> MADTQYILPNDIGVSSLDCREAFRLLSPTERLYAYHLSRAAWYGGLAVLLQTSPEAPYIYALLSRLFRAQDPDQLRQHALAEGLTEEEYQAFLVYAAGVYSNMGNYKSFGDTKFVPNLPKEKLERVILGSEAAQQHPEEVRGLWQTCGELMFSLEPRLRHLGLGKEGITTYFSGNCTMEDAKLAQDFLDSQNLSAYNTRLFKEVDGEGKPYYEVRLASVLGSEPSLDSEVTSKLKSYEFRGSPFQVTRGDYAPILQKVVEQLEKAKAYAANSHQGQMLAQYIESFTQGSIEAHKRGSRFWIQDKGPIVESYIGFIESYRDPFGSRGEFEGFVAVVNKAMSAKFERLVASAEQ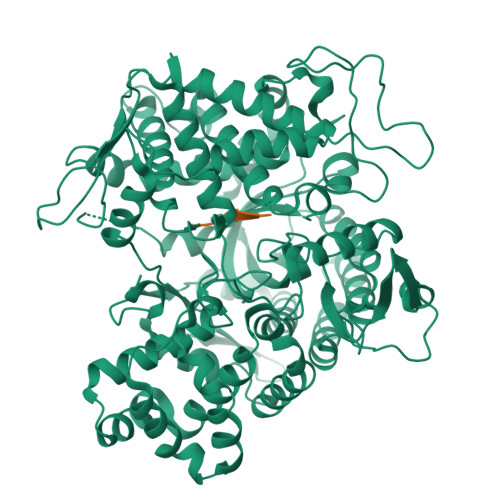LLKELPWPPTFEKDKFLTPDFTSLDVLTFAGSGIPAGINIPNYDDLRQTEGFKNVSLGNVLAVAYATQREKLTFLEEDDKDLYILWKGPSFDVQVGLHALLGHGSGKLFVQDEKGAFNFDQETVINPETGEQIQSWYRSGETWDSKFSTIASSYEECRAESVGLYLCLHPQVLEIFGFEGADAEDVIYVNWLNMVRAGLLALEFYTPEAFNWRQAHMQARFVILRVLLEAGEGLVTITPTTGSDGRPDARVRLDRSKIRSVGKPALERFLRRLQVLKSTGDVAGGRALYEGYATVTDAPPECFLTLRDTVLLRKESRKLIVQPNTRLEGSDVQLLEYEASAAGLIRSFSERFPEDGPELEEILTQLATADARFW;> VVYPW>MVVAHFIVGNTYPYTVSNWEEDIQDAIAVGIDGFALNMGSDAWQVERIEDAYDAAASVSSDFKLFISFDMSIISADADFIEGVVRRFADKPNQLYYDGKVFVSTFAGETDTFGYSDVSTGWDSAVKEPLASAGYPIYFVPSWTSLGQGALEESVADGFLSWNAWPTTDADMNDNDDIGYQNLANSLGKLYVAPVSPWFYTHLSYKNWAYKSDWLIIDRWNEMLSVQPDMIEVLTWNDYGESHYIGNIQGALPAGSEGYVDGFDHTAWRYLMSPYISAYKL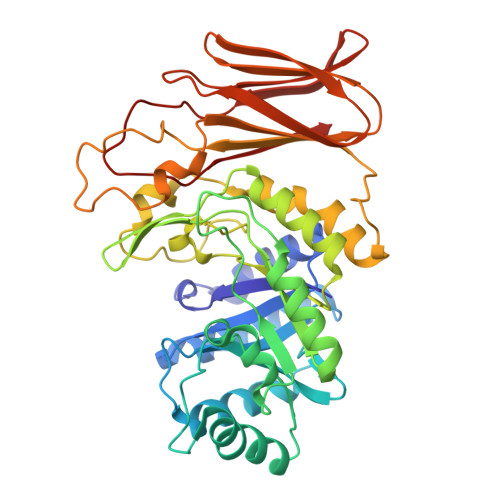GLSEPYINFESLFYWYRPTPKSATATADSLSYPSGGDYMEDEIFVLVYLLQSAEVTVTCGSTTQTFSGVPGVNQFTIPMETNASPSFTVARQGGTLASGTGPEIVDSLSIYNFNAYTGVLYF[3x]>MAQSKHGLTKEMTMKYRMEGCVDGHKFVITGEGIGYPFKGKQAINLCVVEGGPLPFAEDILSAAFNYGNRVFTEYPQDIVDYFKNSCPAGYTWDRSFLFEDGAVCICNADITVSVEENCMYHESKFYGVNFPADGPVMKKMTDNWEPSCEKIIPVPKQGILKGDVSMYLLLKD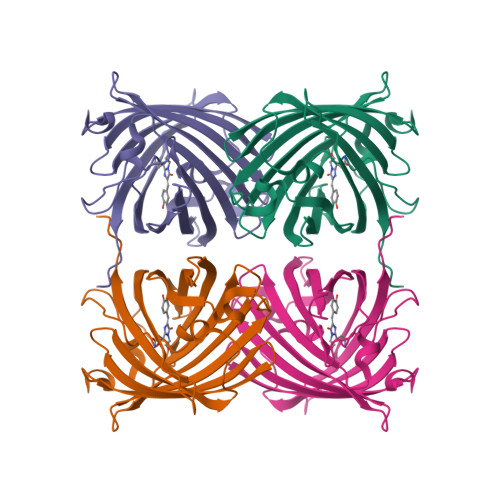GGRLRCQFDTVYKAKSVPRKMPDWHFIQHKLTREDRSDAKNQKWHLTEHAIASGSALP[2x]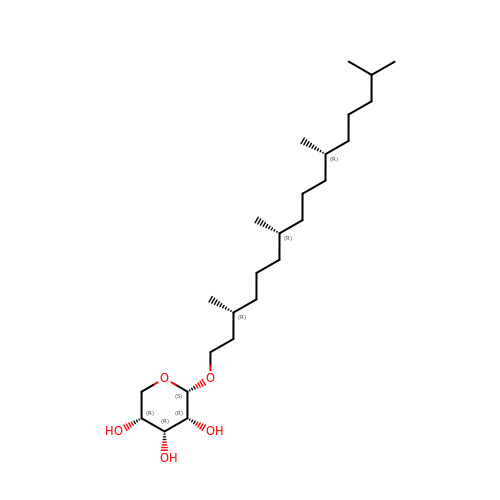(3R,7R,11R)-3,7,11,15-tetramethylhexadecyl alpha-D-ribopyranoside | C25 H50 O5 | ZSTFWXWLAGSUTP-RJQIIPCNSA-N> 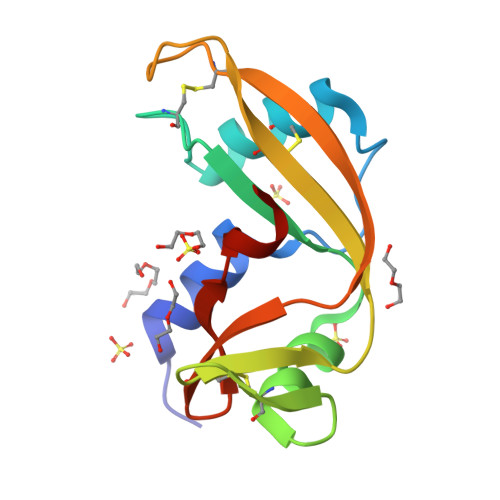MQDNSRYTHFLTQHYDAKPQGRDDRYCESIMRRRGLTSPCKDINTFIHGNKRSIKAICENKNGNPHRENLRISKSSFQVTTCKLHGGSPWPPCQYQATAGFRNVVVACENGLPVHLDQSIFRRP>[3x]DEIGDAAKKLGDASYAFAKEVDWNNGIFLQAPGKLQPLEALKAIDKMIVMGAAADPKLLKAAAEAHHKAIGSISGPNGVTSRADWDNVNAALGRVIASVPENMVMDVYDSVSKITDPKVPAYMKSLVNG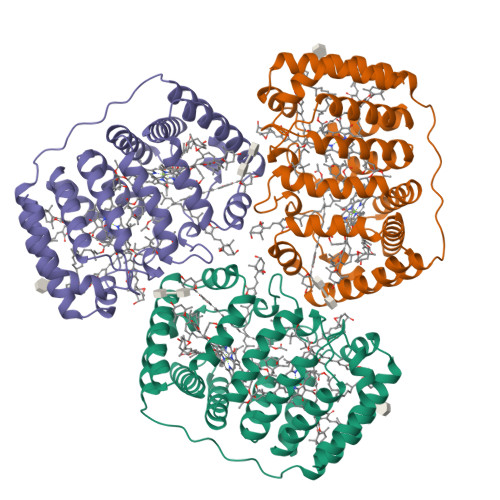ADAEKAYEGFLAFKDVVKKSQVTSAAGPATVPSGDKIGVAAQQLSEASYPFLKEIDWLSDVYMKPLPGVSAQQSLKAIDKMIVMGAQADGNALKAAAEAHHKAIGSIDATGVTSAADYAAVNAALGRVIASVPKSTVMDVYNAMAGVTDTSIPLNMFSKVNPLDANAAAKAFYTFKDVVQAAQ>[2x]CPRFLKVKNWETDVVLTDTLHLKSTLETGCTEHICMGSIMLPSQHTRKPEDVRTKDQLFPLAKEFLDQYYSSIKRFGSKAHMDRLEEVNKEIESTSTYQLKDTELIYGAKHAWRNASRCVGRIQWSKLQVFDARDCTTAHGMFNYICNHVKYATNKGNLRSAITIFPQRTDGKHDFRVWNSQLIRYAGYKQPDGSTLGDPANVQFTEICIQQGWKAPRGRFDVLPLLLQANGNDPE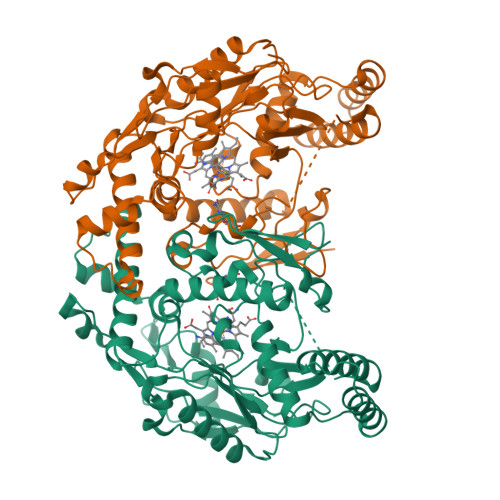LFQIPPELVLEVPIRHPKFDWFKDLGLKWYGLPAVSNMLLEIGGLEFSACPFSGWYMGTEIGVRDYCDNSRYNILEEVAKKMDLDMRKTSSLWKDQALVEINIAVLYSFQSDKVTIVDHHSATESFIKHMENEYRCRGGCPADWVWIVPPMSGSITPVFHQEMLNYRLTPSFEYQPDPWNTHVWKG>[2x]EQARPADDALAALGAQLFVDPALSRNATQSCATCHDPARAFTDPREGKAGLAVSVGDDGQSHGDRNTPTLGYAALVPAFHRDANGKYKGGQFWDGRADDLKQQAGQPMLNPVEMAMPDR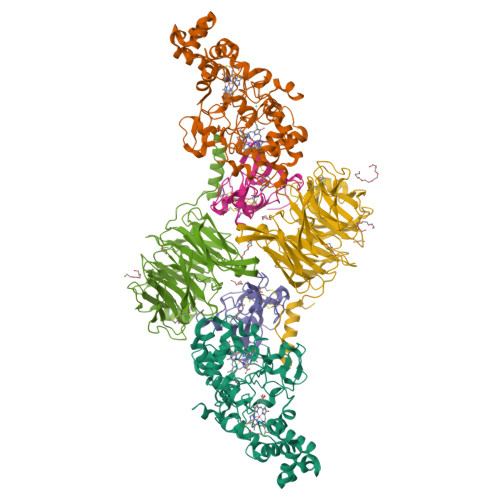AAVAARLRDDPAYRTGFEALFGKGVLDDPERAFDAAAEALAAYQATGEFSPFDSKYDRVMRGEEKFTPLEEFGYTVFITWNCRLCHMQRKQGVAERETFTNFEYHNIGLPVNETAREASGLGADHVDHGLLARPGIEDPAQSGRFKVPSLRNVAVTGPYMHNGVFTDLRTAILFHNKYTSRRPEAKINPETGAPWGEPEVARNLSLAELQSGLMLDDGRVDALVAFLETLTDRRYEPLLEESRAAQKDHHHHHH;>ADAPAGTDPRAKWVPQDNDIQACDYWRHCSIDGNICDCSGGSLTNCPPGTKLATASWVASCYNPTDGQSYLIAYRDCCGYNVSGRCPCLNTEGELPVYRPEFANDIIWCFGAEDDAMTYHCTISPIVGKASHHHHHH[2x];>QDAPEAETQAQETQGQAAARAAAADLAAGQDDEPRILEAPAPDARRVYVNDPAHFAAVTQQFVIDGEAGRVIGMIDGGFLPNPVVADDGSFIAHASTVFSRIARGERTDYVEVFDPVTLLPTADIELPDAPRFLVGTYPWMTSLTPDGKTLLFYQFSPAPAVGVVDLEGKAFKRMLDVPDCYHIFPTAPDTFFMHCRDGSLAKVAFGTEGTPEITHTEVFHPEDEFLINHPAYSQKAGRLVWPTYTGKIHQIDLSSGDAKFLPAVEALTEAERADGWRPGGWQQVAYHRALDRIYLLVDQRDEWRHKTASRFVVVLDAKTGERLAKFEMGHEIDSINVSQDEKPLLYALSTGDKTLYIHDAESGEELRSVNQLGHGPQVITTADMG[2x]>[2x]MGQSKKLNKQPSSLSPLVQLAGIRKCFDGKEVIPQLDLTINNGEFLTLLGPSGCGKTTVLRLIAGLETVDSGRIMLDNEDI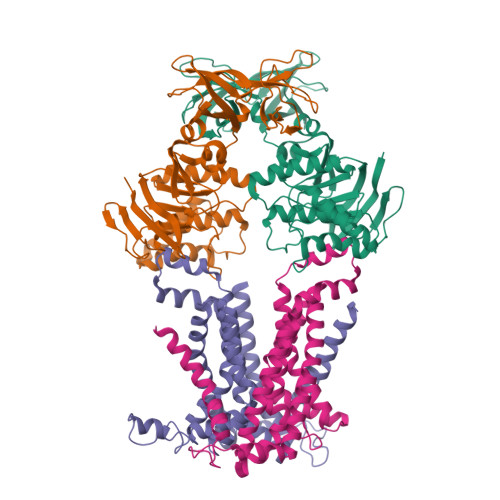THVPAENRYVNTVFQSYALFPHMTVFENVAFGLRMQKTPAAEITPRVMEALRMVQLETFAQRKPHQLSGGQQQRVAIARAVVNKPRLLLLDESLSALDYKLRKQMQNELKALQRKLGITFVFVTHDQEEALTMSDRIVVMRDGRIEQDGTPREIYEEPKNLFVAGFIGEINMFNATVIERLDEQRVRANVEGRECNIYVNFAVEPGQKLHVLLRPEDLRVEEINDDNHAEGLIGYVRERNYKGMTLESVVELENGKMVMVSEFFNEDDPDFDHSLDQKMAINWVESWEVVLADEEHK;> MKNTSKFQNVVIVTIVGWLVLFVFLPNLMIIGTSFLTRDDASFVKMVFTLDNYTRLLDPLYFEVLLHSLNMALIATLACLVLGYPFAWFLAKLPHKVRPLLLFLLIVPFWTNSLIRIYGLKIFLSTKGYLNEFLLWLGVIDTPIRIMFTPSAVIIGLVYILLPFMVMPLYSSIEKLDKPLLEAARDLGASKLQTFIRIIIPLTMPGIIAGCLLVMLPAMGLFYVSDLMGGAKNLLIGNVIKVQFLNIRDWPFGAATSITLTIVMGLMLLVYWRASRLLNKKVELE;> MIGRLLRGGFMTAIYAYLYIPIIILIVNSFNSSRFGINWQGFTTKWYSLLMNNDSLLQAAQHSLTMAVFSATFATLIGSLTAVALYRYRFRGKPFVSGMLFVVMMSPDIVMAISLLVLFMLLGIQLGFWSLLFSHITFCLPFVVVTVYSRLKGFDVRMLEAAKDLGASEFTILRKIILPLAMPAVAAGWVLSFTLSMDDVVVSSFVTGPSYEILPLKIYSMVKVGVSPEVNALATILLVLSLVMVIASQLIARDKTKGNTGDVK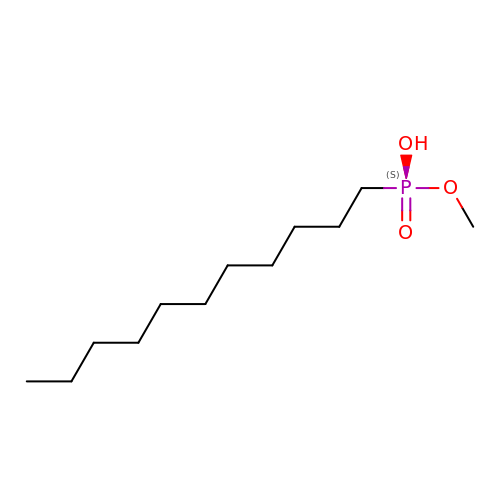METHOXYUNDECYLPHOSPHINIC ACID | C12 H27 O3 P | JBVUSHKPEBKWQP-UHFFFAOYSA-N>[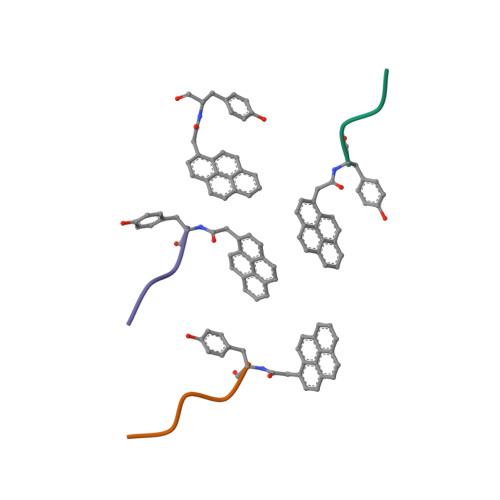4x]XYSPTSPS> MERAEILGVGTELLYGETLDTNTAEIARSLKPYALKVERTLRVADEVAPLAREVEEAFARARLVVLSGGLGPTPDDVTREAVALALGEPLELDEAVLGEIEAFFRARGRAMPEANRKQAMRIPSATWLKNPRGTAPGWWVRKGGKDLVLLPGPPPEWRPMWQEVLPRLGLPRRPYAERVLKTWGIGESEIVERLGPLFVREEEVEVGTYPKVHGVEVVVRGREDRVAELAERIKKKLLKEVWGEGEMTLAEAVKRR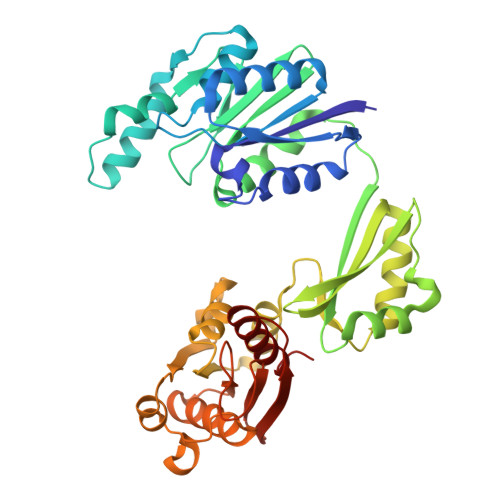MEREGATLSTMESLTGGLLGAEITRVPGASRFYLGGVVSYSVGAKARFGVPQDLLSRTVSAETARAMAEAARSLFGSTYALATTGVAGPDPLEGEPPGTVYVALAGPTGAEVRRYRFPGDRETVRLRSVYAALALLVT>GPMFQRSTPAITLESPDIKYPLRLIDREIISHDTRRFRFALPSPQHILGLPVGQHIYLSARIDGNLVVRPYTPISSDDDKGFVDLVIKVYFKDTHPKFPAGGKMSQYLESMQIGDTIEFRGPSGLLVYQGKGKFAIRPDKKSNPIIRTVKSVGMIAGGTGITPMLQVIRAIMKDPDDHTVCHLLFANQTEKDILLRPELEELRNKHSARFKLWYTLDRAPEAWDYGQGFVNEEMIRDHLPPPEEEPLVLMCGPPPMIQYACLPNLDHVGHPTERCFVF[5x]

Ubiquitin-fold modifier 1 (UFM1) is a UBL covalently conjugated with intracellular proteins through ufmylation, a reaction analogous to ubiquitylation. Here we identify a UFM1 substrate, NADH-cytochrome b5 reductase 3 (CYB5R3), that localizes on the ER membrane. Ufmylation of CYB5R3 depends on the E3 components UFL1 and UFBP1 on the ER, and converts CYB5R3 into its inactive form. Ufmylated CYB5R3 is recognized by UFBP1 through the UFM1-interacting motif, which plays an important role in the further uyfmylation of CYB5R3.

CYB5R3 consists of an N-terminal long hydrophobic stretch sufficient to tightly anchor to the ER, and also FAD- and NADH-binding domains. CYB5R3 catalyzes the transfer of reducing equivalents from NADH to cytochrome b5, which then acts as an electron donor. High-speed atomic force microscopy (HS-AFM) showed that two globular lobes of CYB5R3, which corresponds to the NADH and FAD domains, sometimes separated. All histograms from the data of 6 molecules were well fitted to double-Gaussian distribution whose peaks were at 2.3–2.9 nm (1st peak) and 4.2–5.1 nm (2nd peak). This suggests that CYB5R3 can adopt an open conformation with the two domains distanced from each other. We manually modeled an open conformation of CYB5R3 by changing the arrangement between NADH and FAD domains at the hinge region (Leu147) so that it gives a predicted AFM image similar to the experimental one. The distance between the two lobes of the simulated open conformation was 4.0–4.7 nm, consistent with the value of the 2nd peak of the histogram obtained from the HS-AFM experiment. Since Lys214, the conjugation site for UFM1, was positioned at the interface between the NADH and FAD domains, its ufmylation would bias the equilibrium between closed and open conformations toward the open one, leading to the destruction of the FAD-binding groove and thereby reducing the enzymatic activity of CYB5R3. Remarkably, while free purified CYB5R3 exhibited a brilliant yellow color, the conjugated form was clear. Since FAD emits yellow-green fluorescence, these results indicate that FAD is released from CYB5RC by UFM1 conjugation. Thus, the conjugated form completely lost its reductase activity.> MGSMDQSIAVKSPLTYAEALANTIMNTYTVEELPPANRWHYHQGVFLCGVLRLWEATGEKRYFEYAKAYADLLIDDNGNLLFRRD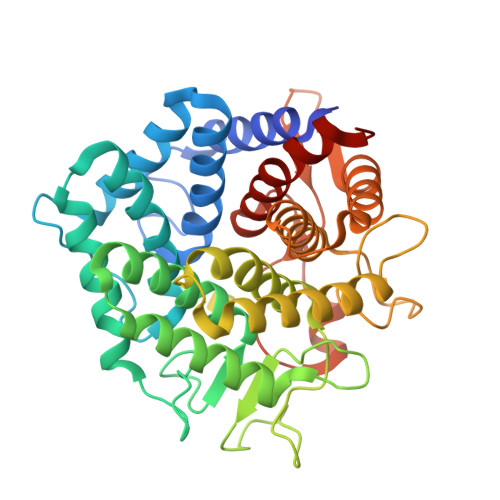ELDAIQAGLILFPLYEQTKDERYVKAAKRLRSLYGTLNRTSEGGFWHKDGYPYQMWLDGLYMGGPFALKYANLKQETELFDQVVLQESLMRKHTKDAKTGLFYHAWDEAKKMPWANEETGCSPEFWARSIGWYVMSLADMIEELPKKHPNRHVWKNTLQDMIKSICRYQDKETGLWYQIVDKGDRSDNWLESSGSCLYMYAIAKGINKGYLDRAYETTLLKAYQGLIQHKTETSEDGAFLVKDICVGTSAGFYDYYVSRERSTNDLHGAGAFILAMTELEPLFRSAGK(2R)-5-[(carbamoyloxy)methyl]-2-{(1S)-1-methoxy-2-oxo-1-[(thiophen-2-ylacetyl)amino]ethyl}-3,6-dihydro-2H-1,3-thiazine-4-carboxylic acid | C16 H19 N3 O7 S2 | 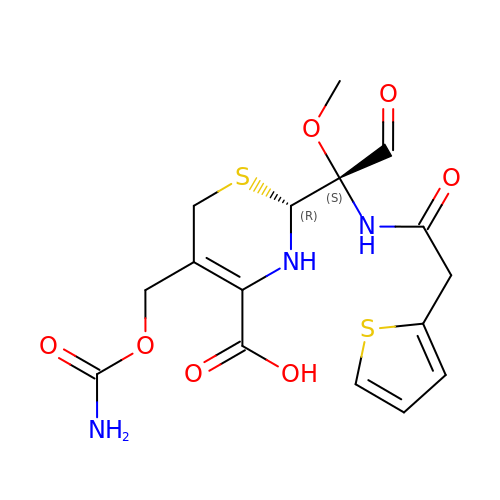IYZWSAWEHPQLHS-ZBFHGGJFSA-N>MIGRLRGIIIEKQPPLVLIEVGGVGYEVHMPMTCFYELPEAGQEAIVFTHFVVREDAQLLYGFNNKQERTLFKELIKTNGVGPKLALAILSGMSAQQFVNAVEREEVGALVKLPGIGKKTAERLIVEMKDRFKGLHGD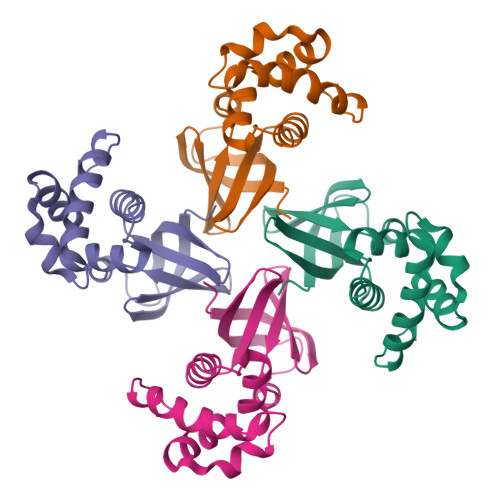LFTPAADLVLT[2x]>GILELAGTVGCVGPRTPIAYMKYGCFCGLGGHGQPRD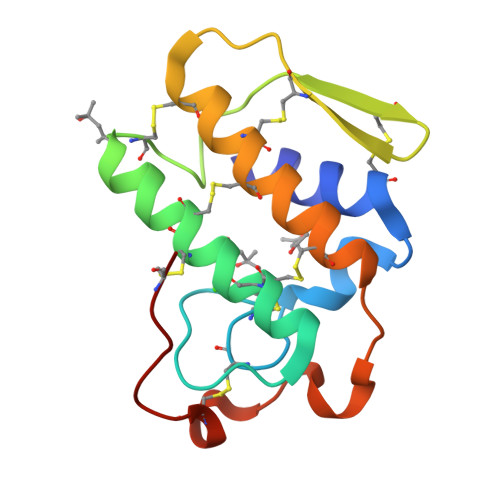AIDWCCHGHDCCYTRAEEAGCSPKTERYSWQCVNQSVLCGPAENKCQELLCKCDQEIANCLAQTEYNLKYLFYPQFLCEPDSPKCD[2x]>MPEIRLRHVVSCSSQDSTHCAENLLKADTYRKWRAAKAGEKTISVVLQLEKE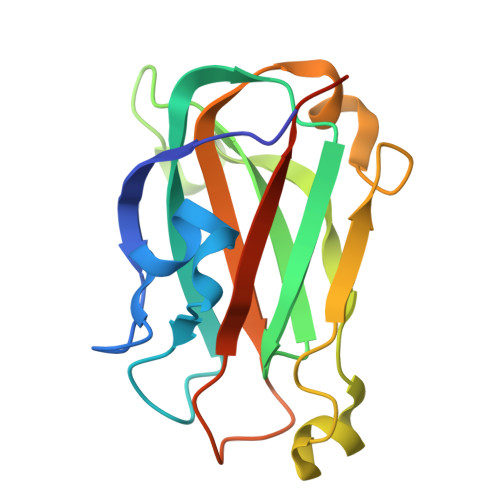EQIHSVDIGNDGSAFVEVLVGSSAGGAGEQDYEVLLVTSSFMSPSESRSGSNPNRVRMFGPDKLVRAAAEKRWDRVKIVCSQPYSKDSPFGLSFVRFHSPPDKHHHHHH[8x]> SSTQIGGMSLDQARTQLAPWTQRAAPIGADEYQQRIERARVLMRAQGVDALLIGAGTSLRYFSGVPWGASERLVALLLTTEGDPVLICPAFEEGSLDAVLQLPVRKRLWEEHEDPYALVVQAMDEQHAHALALDPGIAFAVHTGLRAHLGTAIRDAGAIIDGCRMCKSPAELALMQQACDMTLLVQRLAAGIAHEGIGTDQLVRFIDEAHRALGADNGSTFCIVQFGHATAFPHGIPGVQHLRAGELVLIDTGCTVQGYHSDITRTWIYGTPSDAQQRIWELELAAQAAA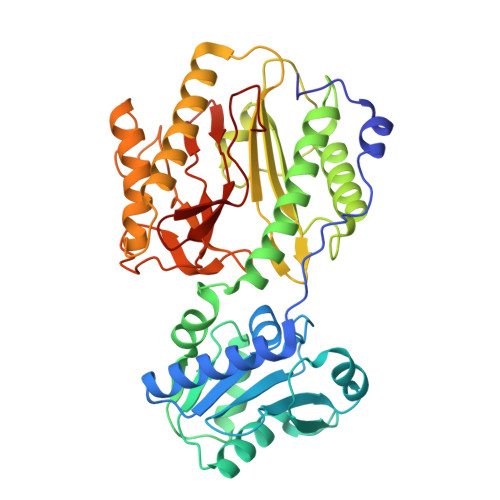FAAVRPGVACEAVDQAARAVLQAAGLGPDYRLPGLPHRTGHGCGLAIHEAPYLVRGNRQPLQPGMCASNEPMIVVPGAFGVRLEDHFYVTDTGAQWFTPPSVAIDQPFA>GPGSRYPVRRLPFSTVSKQDLAAFERIVPGGVVTDPEALQAPNVDWLRTLRGCSKVLLRPRTSEEVSHILRHCHERNLAVNPQGGNTGMVGGSVPVFDEIILSTARMNRVLSFHSVSGILVCQAGCVLEELSRYVEERDFIMPLDLGAKGSCHIGGNVATNAGGLRFLRYGSLHGTVLGLEVVLADGTVLDCLTSLRKDNTGYDLKQLFIGSEGTLGIITTVSILCPPKPRAVNVAFLGCPGFAEVLQTFSTCKGMLGEILSAFEFMDAVCMQLVGRHLHLASPVQESPFYVLIETSGSNAGHDAEKLGHFLEHALGSGLVTDGTMATDQRKVKMLWALRERITEALSRDGYVYKYDLSLPVERLYDIVTDLRARLGPHAKHVVGYGHLGDGNLHLNVTAEAFSPSLLAAL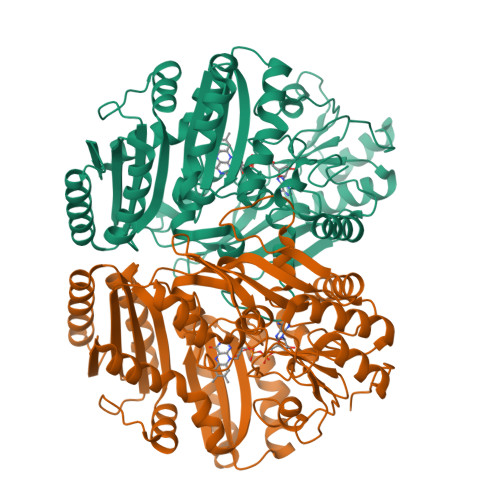EPHVYEWTAGQQGSVSAEHGVGFRKRDVLGYSKPPGALQLMQQLKALLDPKGILNPYKTLPSQAHHHHHH[2x]> KGLENPLPERPREKEEPVVRETGEVVDCHLSDMLQQLHSVNASKPSERGLVRQEEAEDPACIPIFWVSKWVDYSDKYGLGYQLCDNSVGVLFND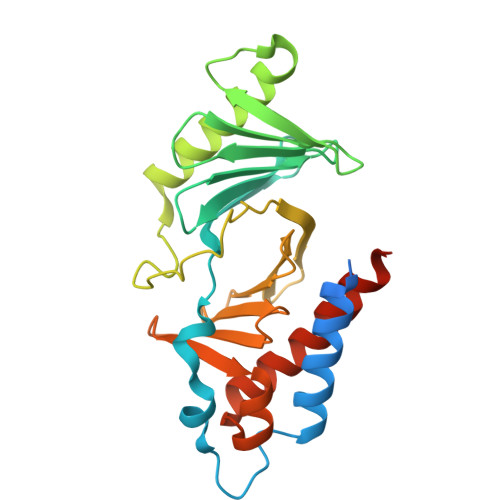STRLILYNDGDSLQYIERDGTESYLTVSSHPNSLMKKITLLKYFRNYMSEHLLKAGANITPREGDELARLPYLRTWFRTRSAIILHLSNGSVQINFFQDHTKLILCPLMAAVTYIDEKRDFRTYRLSLLEEYGCCKELASRLRYARTMVDKLLSSRSASNRLKAS> MRTQCSRALYGRSERGLYFPINHRIVDQRNTLGSGAEEADIQSRYRRQLRSSFVTRETRQTEPPAWSR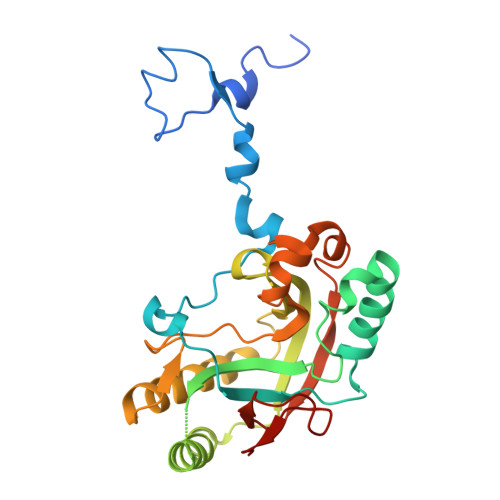STRPTHFLSLPLPARCTLRVRVKEMHESMIFANQSIEPLLIPAAKLHVTLGVMTIGGEMVTAEAVSAAAAPDVLAAIQDCVGQACHDTCKEPLQLRFRGLGTFAHGRVLFAGCITEAHFTTLDTLVRRIRRDVGLGLGVDMKGNPHDSYVPHVTVAKIRPSQIGQFGRQLPISMWADHQHHDFGDVTFNRVDLCSMKGEGKDGYYHVVSSIAVQ>MSIPKSCEVLVAGGGPAGSYAASALAREGVDVVLLEADKHPRYHIGESMLPSIRPLLRFIDLEETFEKHGFQKKLGAAFKLTAKREGYTDFVAAHGPNGYSWNVVRSESDELLFKHAAKSGALTFQGVKVDSLEFEPYDSDFPSGGKVANPGRPVAARWSAKDGRSGTISFQYLVDATGRAGITSTKYLKNRKFNEGLKNLAIWGYYKGARPWAEGTPRENQPYFEGMRDGAGWCWTIPLHNGTVSVGAVLRSDLFFAKKKSLGEDVTNAMIMAECMKLCPTIKELLEPAELVSDIKQATDYSYSASAYAGPYFRIVGDAGCFIDPFFSSGHHLAMAGALAAAVSIRASMKGDCSEYEASNWHARKVDEGYTLFLLVVMAALKQIRMQEEPVLSDIDDDGFDRAFQFLKPVIQGSGSAEIVKRFTKKEVSEAIDFAVLALDNMAGAGEHANETNGSNGTGETNGDAKTLENITVEDEKVLSGIRILAKVAPSADMKDLEGTAIDGFMPRLEHGHLGLNRV[2x]

In particular, the fungal halogenase RadH from Chaetomium chiversii has been shown to be particularly promising in the tailoring of non-tryptophan-derived scaffolds due to the relatively broad range of reactions that can be catalyzed. Based on the study by Menon et al., RadH has demonstrated distinct catalytic activity towards hydroxycoumarin, hydroxyisoquinoline, and phenolic derivatives, in addition to its native substrate Monocillin II. Flavin-dependent halogenases (FDHs) have been pivotal in this domain, given their ability to site-selectively install halogens across a wide range of electron-rich aromatic structures. Our investigation revealed that RadH could effectively halogenate hydroxyquinoline and hydroxybenzothiophene.

Here, a 2.4 Å resolution crystal structure of RadH was obtained using an analogous FDH as a search model, and the crystalline form of this enzyme revealed two largely identical monomers in an asymmetric unit. Each monomer consists of a conserved Flavin-binding domain with FAD bound and a chlorine atom located in an adjacent space. RadH contains several structural features thought to contribute towards the halogenase activity of the enzyme, namely the GxGxxG FAD-binding domain, Fx.Px.Sx.G domain spanning the active site and FAD-binding domain, and a WxWxIP domain on the β-sheet bordering the active site, corroborating similar observations of other FDHs structure. Docking of 6-hydroxyquinoline was performed using DiffDock and suggested that the active site of RadH be the space currently occupied by the flavin moiety of FAD and chlorine atom. While the docked poses overlap with the FAD structure, previous experimental results have shown that nearby residues K74, D325, and F328 are essential for RadH activity, validating the RadH active site proposed by the docking model. The closest structural homolog of RadH is the FAD-dependent chondrochloren halogenase CndH with the lowest RMSD score of 2.39 and 29% sequence identity. Spatial superimposition has revealed highly similar folds between the two proteins, except for an additional omega loop (Y138–P154) in RadH. The binding of carrier proteins is suggested to occur at a hydrophobic groove on CndH next to the entry of the active site. This groove is also where the C-terminus domain of RadH is located (top). As a result, we hypothesize that the C-terminus of RadH has a similar structural role as a docked carrier protein, positioning the enzyme in the correct orientation for catalysis. However, the C-terminus of RadH does not form the full helical lid found in the other variant, A FDHs.>[5x]MGSSHHHHHHSQDPLVPRGSWETEERPR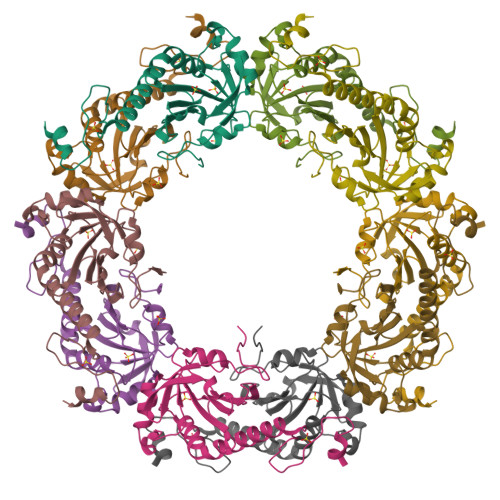TREEEAHFYAGGQVYPGEASRVSVADHSLHLSKAKISKPAPYWEGTAVIDGEFKELKLTDYRGKYLVFFFYPLDFTFVCPTEIIAFGDRLEEFRSINTEVVACSVDSQFTHLAWINTPRRQGGLGPIRIPLLSDLTHQISKDYGVYLEDSGHTLRGLFIIDDKGILRQITLNDLPVGRSVDETLRLVQAFQYTDKHGEVCPAGWKPGSETIIPDPAGKLKYFDKLN>[36x]MPRGSRSAASRPASRPAAPSAHPPAHP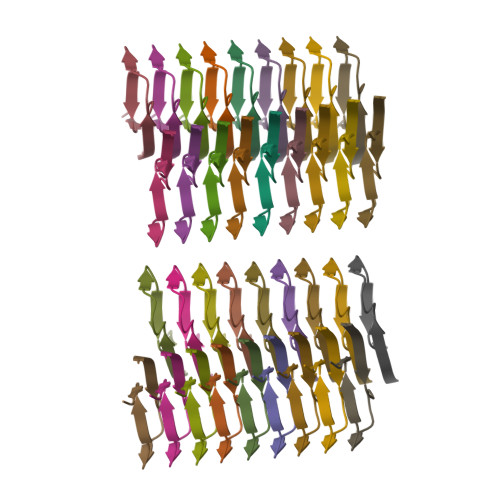PPSAAAPAPAPSGQPGLMAQMATTAAGVAVGSAVGHVMGSALTGAFSGGSSEPSQPAVQQAPTPAAPQPLQ>MSYKLTYFSIRGLAEPIRLFLVDQDIKFIDDRIAKDDFSSIKSQFQFGQLPCLYDGDQQIVQSGAILRHLARKYNLNGENEMETTYIDMFCEGVRDLHVKYTRMIYMAYETEKDPYIKSILPGELAKFEKLLATRGNGRNLILGDKISY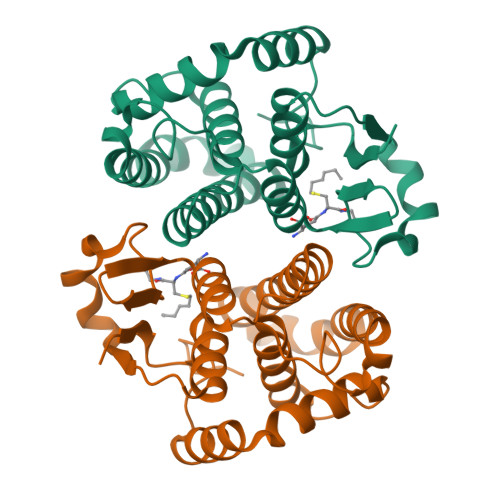ADYALFEELDVHQILDPHCLDKFPLLKVFHQRMKDRPKLKEYCEKRDAAKVPVNGNGKQ[4x]> VHHPPSYVAHLASDFGVRVFQQVAQASKDRNVVFSPYGVASVLAMLQLTTGGETQQQIQAAMGFKIDDKGMAPALRHLYKELMGPWNKDEISTTDAIFVQRDLKLVQGFMPHFFRLFRSTVKQVDFSEVERARFIINDWVKTHTKGMISNLLGKGAVDQLTRLVLVNALYFNGQWKTPFPDSSTHRRLFHKSDGSTVSVPMMAQTNKFNYTEFTTPDGHYYDILELPYHGDTLSMFIAAPYEKEVPLSALTNILSAQLISHWKGNMTRLPRLLVLPK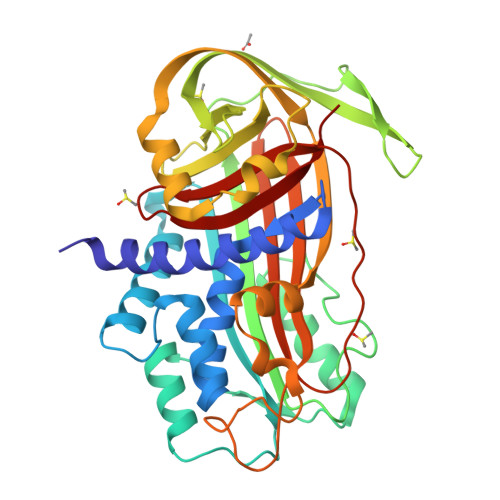FSLETEVDLRKPLENLGMTDMFRQFQADFTSLSDQEPLHVAQALQKVKIEVNESGTVASSSTAVIVSARMAPEEIIMDRPFLFVVRHNPTGTVLFMGQVMEP> KFFEA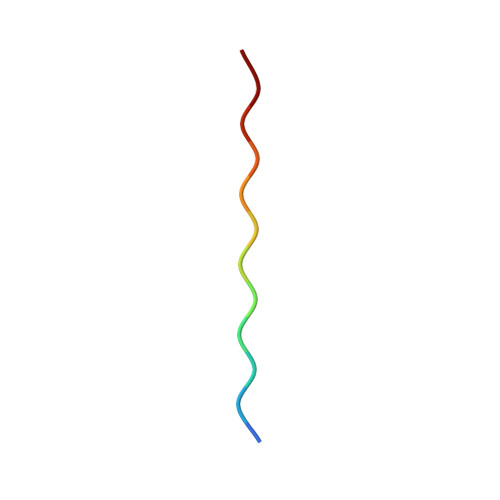AAKKFFE>SNAPPGTV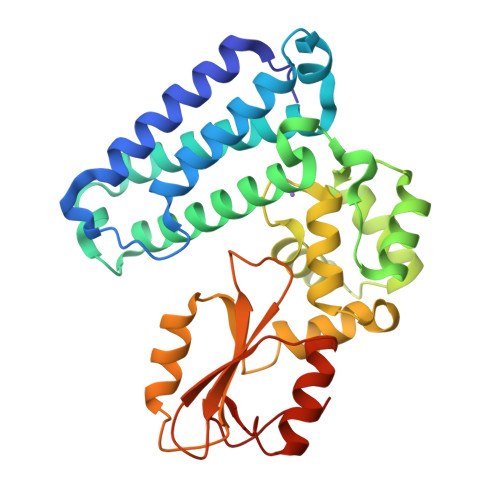DKKMVEKCWKLMDKVVRLCQNPKLALKNSPPYILDLLPDTYQHLRTILSRYEGKMETLGENEYFRVFMENLMKKTKQTISLFKEGKERMYEENSQPRRNLTKLSLIFSHMLAELKGIFPSGLFQGDTFRITKADAAEFWRKAFGEKTIVPWKSFRQALHEVHPISSGLEAMALKSTIDLTCNDYISVFEFDIFTRLFQPWSSLLRNWNSLAVTHPGYMAFLTYDEVKARLQKFIHKPGSYIFRLSCTRLGQWAIGYVTADGNILQTIPHNKPLFQALIDGFREGFYLFPDGRNQNPDLTG[3x]> MIVKHLEEIVDTKDDIDTTTWNSRRLLLTKDGMGFSLNDTLIKAGTETLIWYKNHVEAVYCIEGEGEIEVVGGETYPITPGMMYALDGHEKHYLRARSQMRMVCVFNPPLTG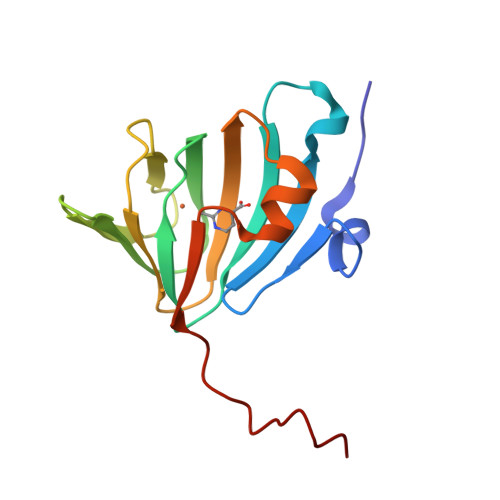AEVHDEEGTYPLLAPITDNWSHPQFE>[2x]ISNEADYDWRNECLRILNLLRKEQNSFLFENPVLESNDLTEETKNRYKEVIPEACDYITIEKRLNNKSNSKRQSTSNQKRKSTTANSKSNQTIENPHEF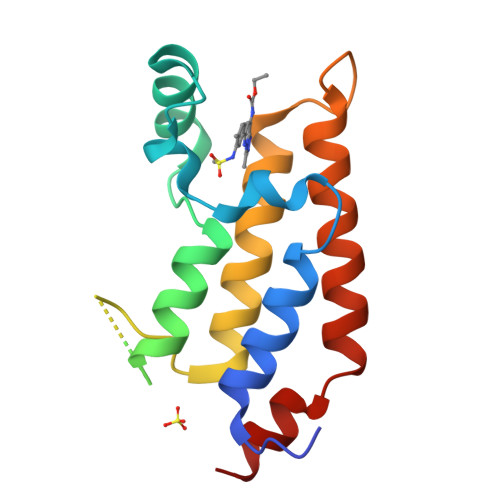ERLVKLIFSNCMIFNPNSGECKWIYDSAKQSLNKFNNLWNKSNVFLLYSNSQ> KLGKLQYSLDYDFQNNQLLVGIIQAAELPALDMGGTSDPYVKVFLLPDKKKKFET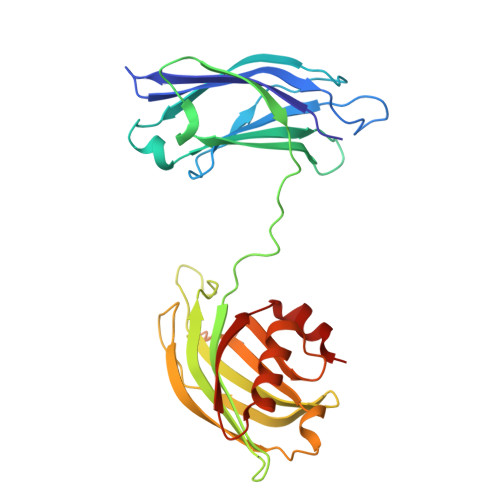KVHRKTLNPVFNEQFTFKVPYSELGGKTLVMAVYDFDRFSKHDIIGEFKVPMNTVDFGHVTEEWRDLQSAEKEEQEKLGDICFSLRYVPTAGKLTVVILEAKNLKKMDVGGLSDPYVKIHLMQNGKRLKKKKTTIKKNTLNPYYNESFSFEVPFEQIQKVQVVVTVLDYDKIGKNDAIGKVFVGYNSTGAELRHWSDMLANPRRPIAQWHTLQVEEEVDAMLAVKK>[2x]MIETTKGGSGSYPIKTIVVLVQENRSFDHTLGWFKELNREIDGVTKSDPKSNTVSSSDTNSLRVVFGDQSQYVNPDPGHSIQDIYEQVFGKPWDSGKPDPNPGHPNMSGFAQNAERNKKGMSSAVMNGFKPNALPVYKELVQNFAICDRWFASVPASTQPNRLYVHSATSHGATSNDAALLLEGFPQKTIFESLDEAGFSFGIYYQFPPSTLFY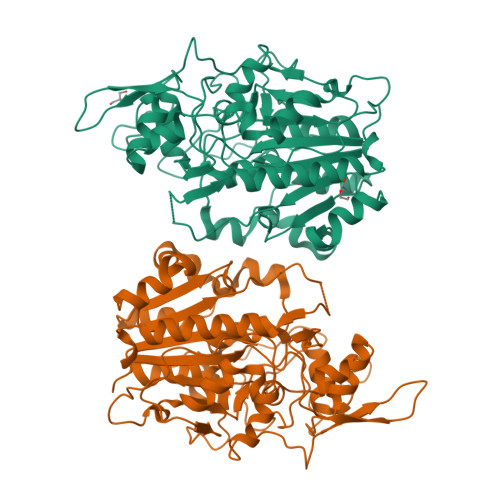RNLRKLKYLTHFHQYGIQFKKDCKEGKLPNYVVVEQRWFDLLSTPANDDHPSHDVSEGQKLVKEVYEALRSSPQWNEILFIITYDEHGGFYDHVPTPVDGVPNPDGILGPPPYNFEFNRLGVRVPTFFISPWIEPGTVIHGPNGPYPRSQYEHSSIPATVKTIFKLKDFLSKRDSWAGTFESVITRDSPRQDCPETLSTPIKLRGTMAKENAQLSEFQEDLVIMAAGLKGDYKNEELIHKLCKETCVADASKYVTNAFEKFLEESRKARDRGCDENDIVY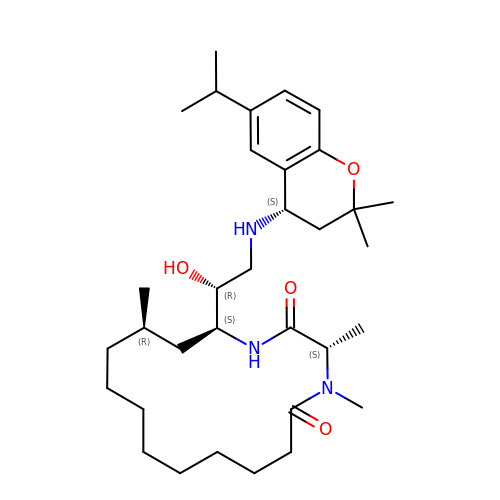(3S,14R,16S)-16-[(1R)-2-{[(4S)-2,2-dimethyl-6-(propan-2-yl)-3,4-dihydro-2H-1-benzopyran-4-yl]amino}-1-hydroxyethyl]-3,4,14-trimethyl-1,4-diazacyclohexadecane-2,5-dione | C33 H55 N3 O4 | MNENNUUKHSBOKZ-BEOVBFIISA-N>ARQSQLSPQNQCQLNQLQAREPDNRIQAEAGQIETWNFNQGDFQCAGVAASRITIQRNGLHLPSYSNAPQLIYIVQGRGVLGAVFSGCPETFEESQQSSQQGRQQEQEQERQQQQQGEQGRQQGQQEQQQERQGRQQGRQQQEEGRQQEQQQGQQGRPQQQQQFRQLDRHQKTRRIREGDVVAIPAGVAYWSYNDGDQELVAVNLFHVSSDHNQLDQNPRKFYLAGNPENEFNQQGQSQPRQQGEQGRPGQHQQPFGRPRQQEQQGNGNNVFSGFNTQLLAQALNVNEETARNLQGQNDNRNQIIQVRGNLDFVQPPRGRQEREHEERQQEQLQQERQQQGEQLMANGLEETFCSLRLKENIGNPERADIFSPRAGRISTLNSHNLPILRF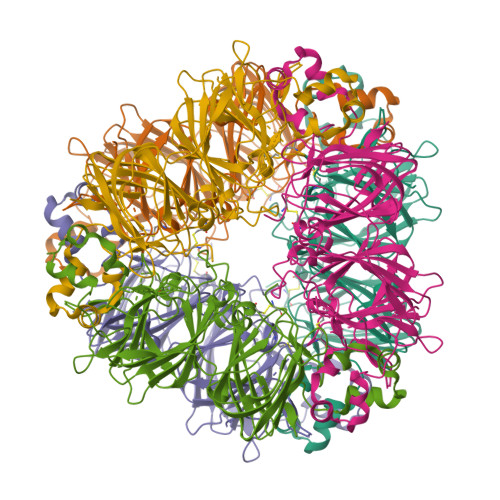LRLSAERGFFYRNGIYSPHWNVNAHSVVYVIRGNARVQVVNENGDAILDQEVQQGQLFIVPQNHGVIQQAGNQGFEYFAFKTEENAFINTLAGRTSFLRALPDEVLANAYQISREQARQLKYNRQETIALSSSQQRRAVV[6x]1,3-dihydroxypropan-2-yl (9Z,12Z)-octadeca-9,12-dienoate | C21 H38 O4 | 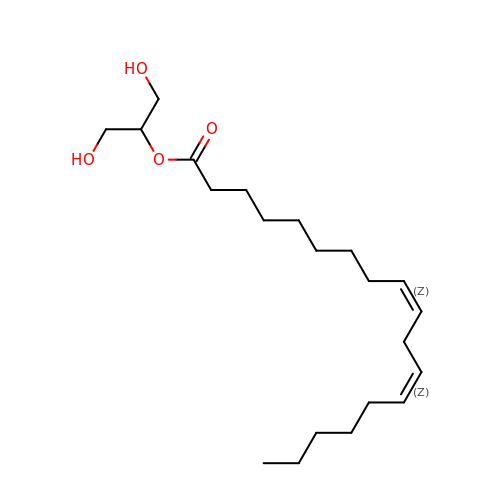IEPGNWMPIFDNSD-HZJYTTRNSA-N Recently, bioinformatics analyses have revealed the presence of CRISPR–Cas loci in bacterial Tn7-like transposons, thereby implicating a functional relationship between RNA-guided DNA targeting and transposition, with the latter representing a new role unrelated to host defense. Support for this concept has emerged from recent functional studies on type I-F and type V-K effectors involved in sequence-specific DNA transposition, thereby significantly broadening the potential biological applications of CRISPR–Cas technology. To complement the available functional studies, our efforts have focused on structural studies of the Vibrio cholerae Tn6677 multi-subunit type I-F CascadecrRNA–TniQ complex, whereby transposition subunit TniQ initiates DNA transposition with the eventual help of other transposition-associated proteins TnsA, TnsB and TnsC in the gene cluster. Here we report cryo-EM structures of a V. cholerae type I-F CascadecrRNA in complex with transposition subunit TniQ before (binary CascadecrRNA–TniQ) and after (ternary CascadecrRNA–TniQ–dsDNA) target double-stranded DNA (dsDNA) binding at an average resolution of 2.9 Å and 3.2 Å, respectively.

Our CascadecrRNA–TniQ–dsDNA ternary complex contains a G–G/C–C PAM (protospacer adjacent motif) sequence, which is required for binding of the target sequence, allowing CRISPR–Cas systems to discriminate between self and non-self. The target sequence contains 12-base pair (bp) of PAM-proximal duplex DNA and 51-bp of PAM-distal duplex DNA. We could observe only 5-bp of PAM-proximal duplex DNA with 2-nt overhang at the 3′ end of the non-target strand (NTS), and a traceable 32-nt target DNA strand complementary and paired to 32-nt spacer RNA, but no clear density for the PAM-distal duplex segment, which is adjacent to bound TniQ. The G–G/C–C PAM is specifically recognized by Ser127 and Asn246 in Cas8. Arg243 forms a wedge and stacks with PAM G (–1), facilitating the formation of crRNA–target DNA heteroduplex and displacing the NTS, thus leading to the onset of R-loop formation. In line with this concept, we observe that TniQ forms a head-to-tail dimer whose individual monomers simultaneously bind to Cas6 and Cas7.1 of the CascadecrRNA complex, with clear density observed at the interface between TniQ and both Cas6 and Cas7.1. One TniQ interacts with Cas6 via a main chain polar interaction between Val268 and Asn16, whereas the other TniQ interacts with Cas7.1 by multiple polar interactions between side chains over a larger interface (inset). Notably, the binary and DNA-bound ternary CascadecrRNA–TniQ complexes superpose with an RMSD of 2.33 Å. Minimal conformational changes are observed on ternary complex formation in the presence of bound target DNA, reflecting slight opening of the entire complex and crRNA, especially within the TniQ-bound end.

> MQTLKELIASNPDDLTTELKRAFRPLTPHIAIDGNELDALTILVNLTDKTDDQKDLLDRAKCKQKLRDEKWWASCINCVNYRQSHNPKFPDIRSEGVIRTQALGELPSFLLSSSKIPPYHWSYSHDSKYVNKSAFLTNEFCWDGEISCLGELLKDADHPLWNTLKKLGCSQKTCKAMAKQLADITLTTINVTLAPNYLTQISLPDSDTSYISLSPVASLSMQSHFHQRLQDENRHSAITRFSRTTNMGVTAMTCGGAFRMLKSGAKFSSPPHHRLNSKRSWLTSEHVQSLKQYQRLNKSLIPENSRIALRRKYKIELQNMVRSWFAMQDHTLDSNILIQHLNHDLSYLGATKRFAYDPAMTKLFTELLKRELSNSINNGEQHTNGSFLVLPNIRVCGATALSSPVTVGIPSLTAFFGFVHAFERNINRTTSSFRVESFAICVHQLHVEKRGLTAEFVEKGDGTISAPATRDDWQCDVVFSLILNTNFAQHIDQDTLVTSLPKRLARGSAKIAIDDFKHINSFSTLETAIESLPIEAGRWLSLYAQSNNNLSDLLAAMTEDHQLMASCVGYHLLEEPKDKPNSLRGYKHAIAECIIGLINSITFSSETDPNTIFWSLKNYQNYLVVQPRSINDETTDKSSL;>MKLPTNLAYERSIDPSDVCFFVVWPDDRKTPLTYNSRTLLGQMEAASLAYDVSGQPIKSATAEALAQGNPHQVDFCHVPYGASHIECSFSVSFSSELRQPYKCNSSKVKQTLVQLVELYETKIGWTELATRYLMNICNGKWLWKNTRKAYCWNIVLTPWPWNGEKVGFEDIRTNYTSRQDFKNNKNWSAIVEMIKTAFSSTDGLAIFEVRATLHLPTNAMVRPSQVFTEKESGSKSKSKTQNSRVFQSTTIDGERSPILGAFKTGAAIATIDDWYPEATEPLRVGRFGVHREDVTCYRHPSTGKDFFSILQQAEHYIEVLSANKTPAQETINDMHFLMANLIKGGMFQHKGD[6x];> MKWYYKTITFLPELCNNESLAAKCLRVLHGFNYQYETRNIGVSFPLWCDATVGKKISFVSKNKIELDLLLKQHYFVQMEQLQYFHISNTVLVPEDCTYVSFRRCQSIDKLTAAGLARKIRRLEKRALSRGEQFDPSSFAQKEHTAIAHYHSLGESSKQTNRNFRLNIRMLSEQPREGNSIFSSYGLSNSENSFQPVPLI;>[2x]MFLQRPKPYSDESLESFFIRVANKNGYGDVHRFLEATKRFLQDIDHNGYQTFPTDITRINPYSAKNSSSARTASFLKLAQLTFNEPPELLGLAINRTNMKYSPSTSAVVRGAEVFPRSLLRTHSIPCCPLCLRENGYASYLWHFQGYEYCHSHNVPLITTCSCGKEFDYRVSGLKGICCKCKEPITLTSRENGHEAACTVSNWLAGHESKPLPNLPKSYRWGLVHWWMGIKDSEFDHFSFVQFFSNWPRSFHSIIEDEVEFNLEHAVVSTSELRLKDLLGRLFFGSIRLPERNLQHNIILGELLCYLENRLWQDKGLIANLKMNALEATVMLNCSLDQIASMVEQRILKPNRKSKPNSPLDVTDYLFHFGDIFCLWLAEFQSDEFNRSFYVSRW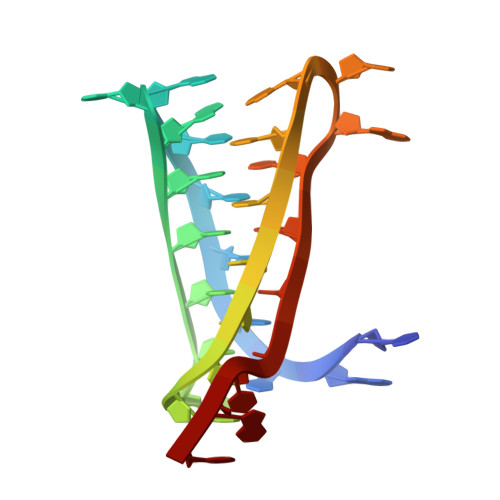>[2x]TATCCCCACACCCCTATCCCCACACCCCTAT> KPRIPVVWIHGLECTCCTESFIRSAHPLAKDVILSLISLDYDDTLMAAAGTQAEEVFEDIITQYNGKYILAVEGNPPLGEQGMFCISSGRPFIEKLKRAAAGASAIIAWGTCASWGCVQAARPNPTQATPIDKVITDKPIIKVPGCPPIPDVMSAIITYMVTFDRLPDVDRMGRPLMFYGQRI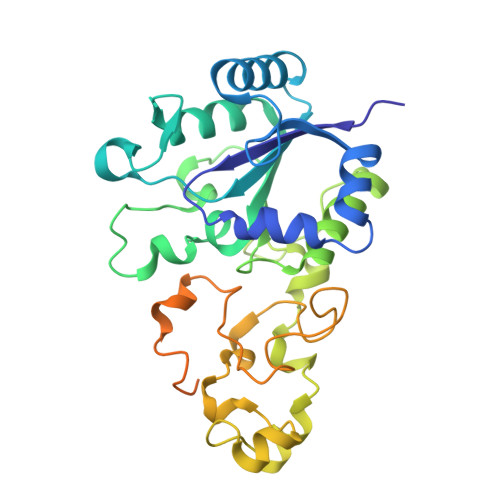HDKCYRRAHFDAGEFVQSWDDDAARKGYCLYKMGCKGPCTYNACSSTRWNDGVSFPIQSGHGCLGCAENGFWDRGSFYSRVVDIPQMGTHSTADTVGLTALGVVAAAVGVHAVASAVDQRRRHNQQPTETEHQPGNEDKQA> KLC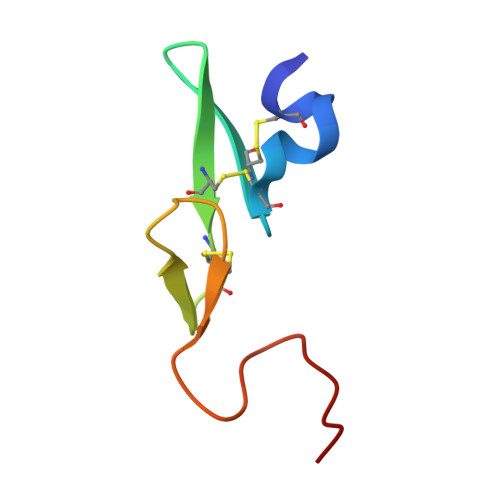SLDNGDCDQFCHEEQNSVVCSCARGYTLADNGKACIPTGPYPCGKQTLE Hydrogen sulfide (H2S) plays roles in many physiological processes in mammals, including relaxation of vascular smooth muscles, regulation of inflammation, and inhibition of insulin signaling. More recently, it has been proposed that sulfane sulfurs, i.e., sulfur atoms with oxidation state 0 or −1, existing in the form of polysulfides (H2Sn), glutathione persulfide (GSSH), glutathione trisulfide (GSSSG), cysteine persulfide (CysSSH) and so on, actually mediate some of the reported biological activities previously thought to be regulated by H2S67891011. We determined the crystal structures of the m3MST complexes with 1 and 3 at high resolution. The most remarkable feature is that C248 is persulfurated in both crystal structures.

Interestingly, 1–3 all have a similar structural scaffold, i.e., an aromatic ring-carbonyl-S-pyrimidone structure. Persulfurated C248 appears to interact with the 4-pyrimidone-like aromatic ring of both compounds. To our knowledge, this interaction is novel in terms of both the long distance (>3.45 Å) and the orientation of the persulfide bond (almost perpendicular to the aromatic ring of the inhibitors). Direct hydrogen bonding by R188 and S250 and water-mediated hydrogen bonding by E195 and R197 are commonly observed with compounds 1 and 3. In addition, compound 1 forms water-mediated hydrogen bonds with D63 and H74. Both compounds were in van der Waals contact with W36, L38, P39, D73, H74, Y108, R188, P196, R197, G249, S250, V252 and V277. The thiophene ring (compound 1) and naphthalene ring (compound 3) exhibit cation-π interaction with R197 and parallel stacking interaction with the salt bridge between D73 and R19726. Gas-phase calculations indicated that the interaction of S–S− with pyrimidone is strongly exothermic (10.4 kcal/mol; CCSD(T)/aug-cc-pVDZ), which is not inconsistent with the experimental ITC measurements (ΔH = −9.37 and −11.76 kcal/mol for compounds 1 and 3, respectively). We concluded that the interaction is predominantly due to electrostatic attraction between the persulfur anion and the positively charged carbonyl carbon of the pyrimidone structure. Compound 1 showed about 25% inhibition of recombinant CBS and CSE enzymatic activities, while compound 3 was almost inactive towards CBS and CSE.

>MAAPQLFRALVSAQWVAEALKAPRSSQPLKLLDASWYLPKLGRDARREFEERHIPGAAFFDIDRSSDHTSPYDHMLPNATHFADYAGSLGVSAATHVVIYDGSDQGLYSAPRVWWMFRAFGHHSVSLLDGGFRHWLNQNLPISSGKSHSEPAEFSAQLDPSFIKTHEDILENLDARRFQVVDARAAGRFQGTQPEPRDGIEPGHIPGSVNIPFTEFLTNEGLEKSPEEIKRLFKEKKVDLSKPLVATCGSGVTASHVVLGAFLSGKSDVPVYDGSWVEWYMRAQPEHIISEGRGKTQ[2x]> MAFKVISQENLLEQKRKETLQEDIPFIVNGEMEYVTKKISNGEMETLELNKPLGEMMTFSSTSNLKELLRKVVLDVELGREQVQLLYKPIYDSIADSNLPQVMDAKWALQGNCVFLEHIEGEEIKFGTINAENGPVARIQTYATGFEYTKEMKDFNQTFSVEILNKSIGESYNALLNHIHLSPIINFNYKASNKTAFKGETNDPIWLGIWRTLTQAQKDTVIAKRQGNILMASSADQIEIEMALNGGHLLNGSMYPSIKNISTVIYYDGWEVTVGKKTYSYKGVTPGKGYLIRPKRGFKELIKRDLTT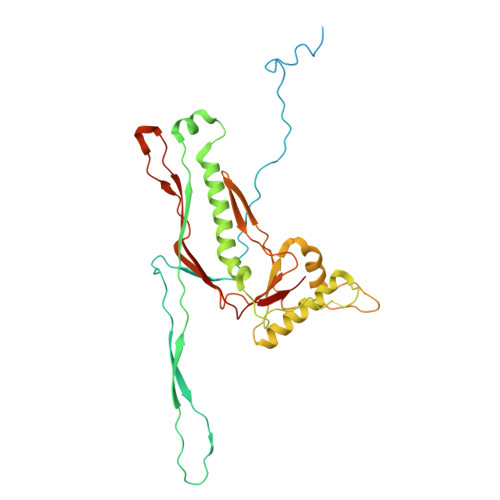EVGNADLSKLVENQIVGHCYRGAFAAVEENVQEISFR5'-deoxy-5'-[({5-[(3aS,4S,6aR)-2-oxohexahydro-1H-thieno[3,4-d]imidazol-4-yl]pentanoyl}sulfamoyl)amino]adenosine 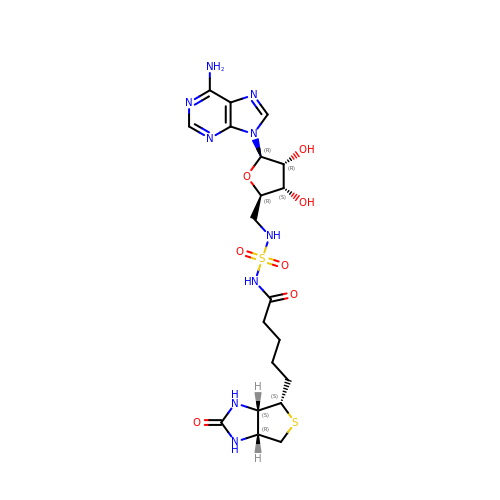| C20 H29 N9 O7 S2 | RSZBCKJLQVSFKT-RHCAYAJFSA-N(3~{S},7~{R},10~{R},13~{R})-4-[(3~{S},6~{R},8~{a}~{S})-1'-[(2~{S})-2-acetamido-3-(2-chlorophenyl)propanoyl]-5-oxidanylidene-spiro[1,2,3,8~{a}-tetrahydroindolizine-6,2'-pyrrolidine]-3-yl]carbonyl-2-oxidanylidene-1,4-diazatricyclo[8.3.0.0^{3,7}]tridec-8-ene-13-carboxylic acid | C35 H40 Cl N5 O7 | 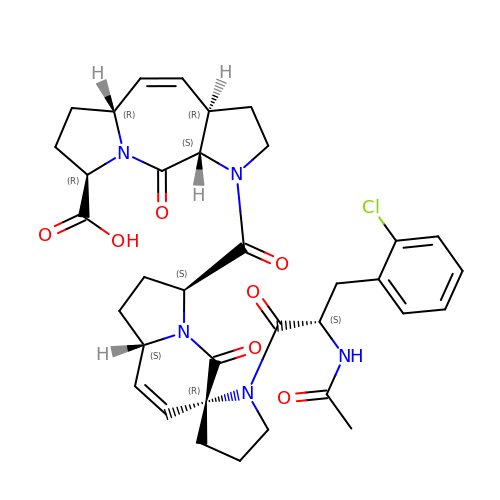AYDUPBNKBXOHLZ-LMFSJQDSSA-N>[2x]MKEKVVSLAQDLIRRPSISPNDEGCQQIIAERLEKLGFQIEWMPFNDTLNLWA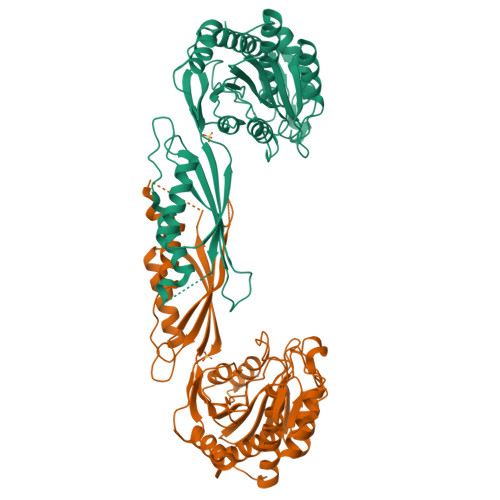KHGTSEPVIAFAGHTDVVPTGDENQWSSPPFSAEIIDGMLYGRGAADMKGSLAAMIVAAEEYVKANPNHKGTIALLITSDEEATAKDGTIHVVETLMARDEKITYCMVGEPSSAKNLGDVVKNGRRGSITGNLYIQGIQGHVAYPHLAENPIHKAALFLQELTTYQWDKGNEFFPPTSLQIANIHAGTGSNNVIPAELYIQFNLRYCTEVTDEIIKQKVAEMLEKHNLKYRIEWNLSGKPFLTKPGKLLDSITSAIEETIGITPKAETGGGTSDGRFIALMGAEVVEFGPLNSTIHKVNECVSVEDLGKCGEIYHKMLVNLLDS> ALDAAETGHTSSVQPEDVIETRYVQTSQTRDEMSLESFLGRSGCIHESKLEVTLANYNKENFTVWAINLQEMAQIRRKFELFTYTRFDSEITLVPCISALSQDIGHITMQYMYVPPGAPVPNSRDDYAWQSGTNASVFWQHG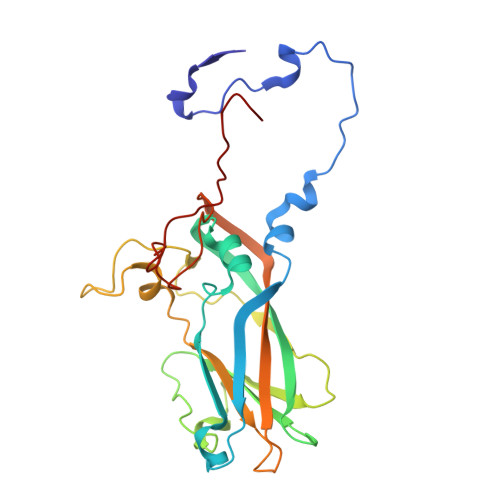QAYPRFSLPFLSVASAYYMFYDGYDEQDQNYGTANTNNMGSLCSRIVTEKHIHKVHIMTRIYHKAKHVKAWCPRPPRALEYTRAHRTNFKIEDRSIQTAIVTRPIITTA SulE, an esterase, which detoxifies a variety of sulfonylurea herbicides through de-esterification, provides an attractive approach to remove environmental sulfonylurea herbicides and develop herbicide-tolerant crops. SulE catalyzes the de-esterification of a variety of sulfonylurea herbicides, such as MM, BM, SM, TM, TrM, EM, and CE, to the corresponding herbicidal-inactive parent acid. The structures show that SulE is a dimer with a lid loop in a domain-swapped β-hairpin covering the active site from the opposing monomer. SulE shows a similar catalytic triad consisting of Ser209, His333, and Glu232 at its active site.

Previously, we obtained a mutant P44R through directed evolution, which showed 1.7- to 3.2- fold improvement in catalytic efficiencies towards MM, SM, CE, TrM, and EM, but showed 0.18- and 0.28-fold decrease in catalytic efficiencies towards BM and TM, respectively. Structural analysis showed that Pro44 is located in the lid loop. To understand the molecular basis for the altered activity by Pro44 mutation, the crystal structures of apo-P44R, the double mutant P44R/S209A in complex with CA, and the triple mutant P44R/S209A/H333A in complex with MM, CE, and TM were determined in the range of 1.32–1.78 Å. Apo-P44R structure is almost identical to the WT apo-SulE structure with an RMSD of 0.17 Å of the aligned Cα. In addition, the B factors of the residues in this loop region is much higher in P44R mutant than in the wildtype, suggesting that the mutation of Pro44 to arginine makes this loop region more flexible. Structural comparison analysis shows that the P44R mutation leads to lid loop shift, which in turn modulates substrate binding and enzyme activity. Structural analysis indicated that the substitution of Pro44 with arginine altered the flexibility of the lid loop, and further allowed the relocation of the heterocycle ring of MM and CE.

>[2x]METDNVELAQSKRKVVLAEQGSFYIGGRTVTGPGKFDPSKPVIRYSNEGATFYINQMYVNFQAPVRPRGLPLVFWHGGGLTGHIWESTPDGRPGFQTLFVQDRHTVYTIDQPGRGRGNIPTFNGPFGQLEEESIVNTVTGNSSKEGAWVRDRLGPAPGQFFENSQFPRGYEDNYFKEMGFSPSISSDEIVDAVVKLVTHIGPCVLVTHSASGVLGMRVATHAKNVRGIVAYEPATSIFPKGKVPEIPPLADKKSQIFPPFEIQESYFKKLAKIPIQFVFGDNIPKNPKSAYWFLDWWRVTRYAHSLSLEAINKLGGQASLLDLPTAGLRGNTHFPFTDRNNVQVASLLSDFLGKHGLDQNESLEHHHHHH> SNAMKPTLFVLAAGMGSRYGSLKQLDGIGPGGDTIMDYSVYDAIRAGFGRLVFVIRHSFEKEFREKILTKYEGRIPVELVFQELDRLPEGFSCPEGREKPWGTNHAVLMGRDAIREPFAVINADDFYGRNGFEVLARKLMTLEGKQGEYCMVGYRVGNTLSESGGVS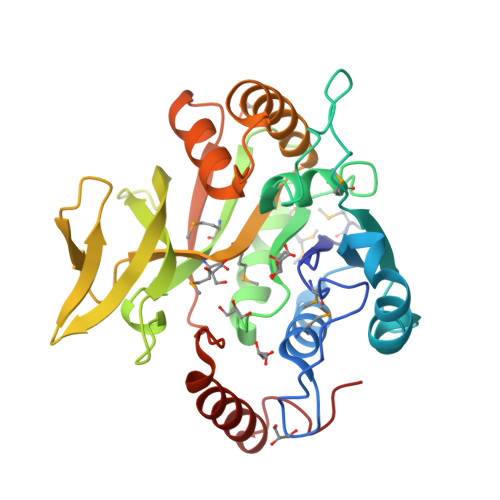RGVCQVDEKHLLTGVVERTGIERTDGTISFRDETGKICTLAEDAPVSMNMWGFTPDYFDYSEELFINFLNAHGQEPKSEFFIPFVVNDLIRSGRASVEVLDTTARWFGVTYSDDRPGVVAKLRELTEAGEYPTKLF>PFINIKLVP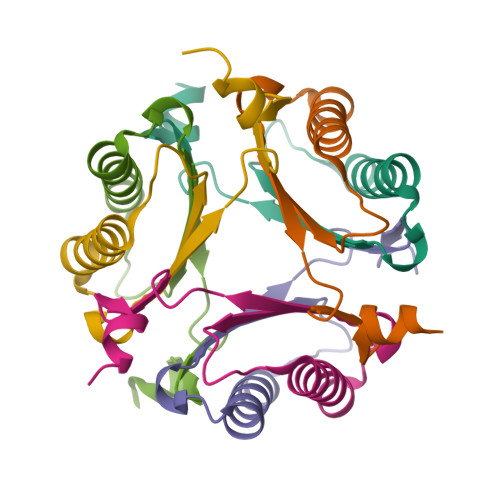ENGGPTNEQKQQLIEGVSDLMVKVLNKNKASIVVIIDEVDSNNYGLGGESVHHLRQKN[6x]>[2x]NSLMSVGYFNGGGDVTAGPGGDIDKLDVRQITHLNYSFGLVYNDEKDETNAALKDPSKLHQIWLSPKVQADLQKIPSLRQQNPNLKVLLSVGGWGARGFSGAAATKETRAVFIQSAQAIIEKYGLDGIDLDWEYPVNGAWGLVASQPADRDNFTALLKELRAAVGNKKLVTIAVGANAESPKSWVDVKAIAPSLDYINLMTYDLAYGTQYFNSNLYDSTRWPTVAEADKYSADFIVNN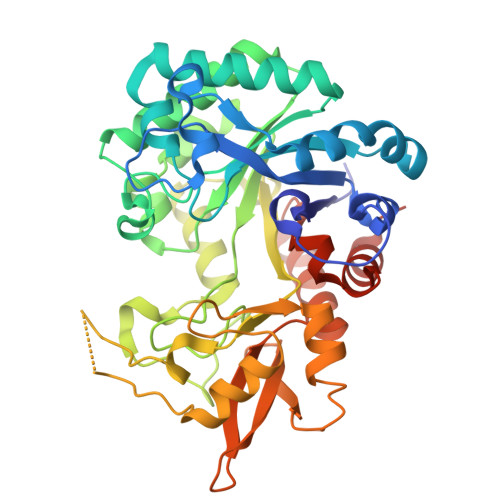YLAAGLKPSQMNLGIGFYGRIPKRAVEPGIDWSKPDAQKNPATRPYFAAQQIELFESLGVDLTKDTYVKYNDIVAKLINDPQKRFTQHWDDEGKVPWLSVQSADGQALFALSYENPRSVAIKADYIKSKGLGGAMFWEYGADDQNQLAKQLAESLGIKRLEHHHHHH>[2x]DFGLDCDEHSTESRCCRYPLTVDFEAFGWD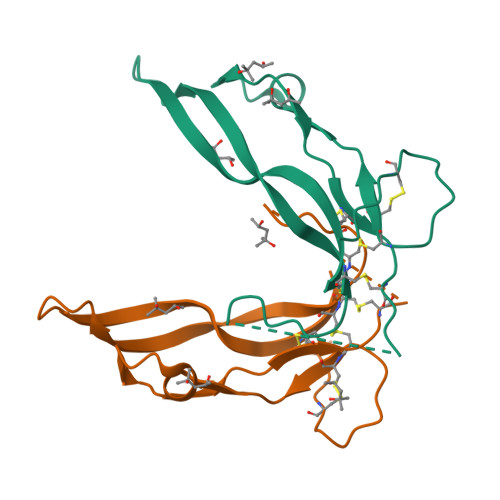WIIAPKRYKANYCSGECEFVFLQKYPHTHLVHQANPRGSAGPCCTPTKMSPINMLYFNGKEQIIYGKIPAMVVDRCGCS>[6x]SNAMENQKMQEPLVYRRILLTVDEDDNTSSERAFRYATTLAHDYDVPLGICSVLESEDINIFDSLTPSKIQAKRKHVEDVVAEYVQLAEQR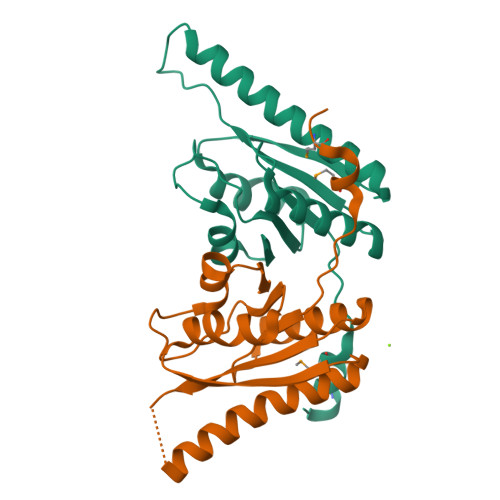GVNQVEPLVYEGGDVDDVILEQVIPEFKPDLLVTGADTEFPHSKIAGAIGPRLARKAPISVIVVR> MATATEQWVLVEMVQALYEAPAYHLILEGILILWIIRLLFSKTYKLQERSDLTVKEKEELIEEWQPEPLVPPVPKDHPALNYNIVSGPPSHKTVVNGKECINFASFNFLGLLDNPRVKAAALASLKKYGVGTCGPRGFYGTFDVHLDLEDRLAKFMKTEEAIIYSYGFATIASAIPAYSKRGDIVFVDRAACFAIQKGLQASRSDIKLFKHNDMADLERLLKEQEIEDQKNPRKARVTRRFIVVEGLYMNTGTICPLPELVKLKYKYKARIFLEESLSFGVLGEHGRGVTEHYGINIDDIDLISANMENALASIGGFCCGRSFVIDHQRLSGQGYCFSASLPPLLAAAAIEALNIMEENPGIFAVLKEKCGQIHKALQGISGLKVVGESLSPAFHLQLEESTGSREQDVRLLQEIVDQCMNRSIALTQARYLEKEEKCLPPPSIRVVVTVEQTEEELERAASTIKEVAQAVLL;> MRPEPGGCCCRRTVRANGCVANGEVRNGYVRSSAAAAAAAAAGQIHHVTQNGGLYKRPFNEAFEETPMLVAVLTYVGYGVLTLFGYLRDFLRYWRIEKCHHATEREEQKDFVSLYQ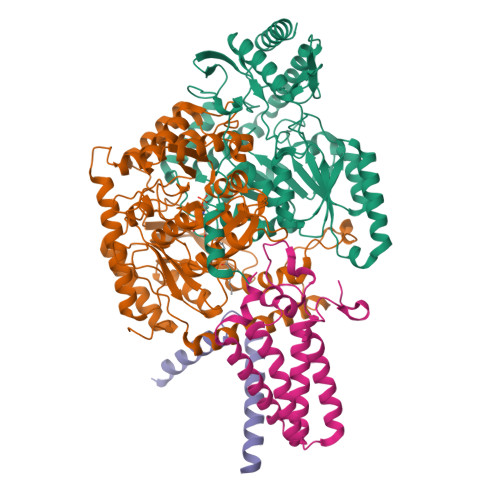DFENFYTRNLYMRIRDNWNRPICSVPGARVDIMERQSHDYNWSFKYTGNIIKGVINMGSYNYLGFARNTGSCQEAAAKVLEEYGAGVCSTRQEIGNLDKHEELEELVARFLGVEAAMAYGMGFATNSMNIPALVGKGCLILSDELNHASLVLGARLSGATIRIFKHNNMQSLEKLLKDAIVYGQPRTRRPWKKILILVEGIYSMEGSIVRLPEVIALKKKYKAYLYLDEAHSIGALGPTGRGVVEYFGLDPEDVDVMMGTFTKSFGASGGYIGGKKELIDYLRTHSHSAVYATSLSPPVVEQIITSMKCIMGQDGTSLGKECVQQLAENTRYFRRRLKEMGFIIYGNEDSPVVPLMLYMPAKIGAFGREMLKRNIGVVVVGFPATPIIESRARFCLSAAHTKEILDTALKEIDEVGDLLQLKYSRHRLVPLLDRPFDETTYEETED;> MAGMALARAWKQMSWFYYQYLLVTALYMLEPWERTVFNSMLVSIVGMALYTGYVFMPQHIMAILHYFEIVQ;> MNVGTAHSEVNPNTRVMNSRGIWLSYVLAIGLLHIVLLSIPFVSVPVVWTLTNLIHNMGMYIFLHTVKGTPFETPDQGKARLLTHWEQMDYGVQFTASRKFLTITPIVLYFLTSFYTKYDQIHFVLNTVSLMSVLIPKLPQLHGVRIFGINKY> MDINDNHPTW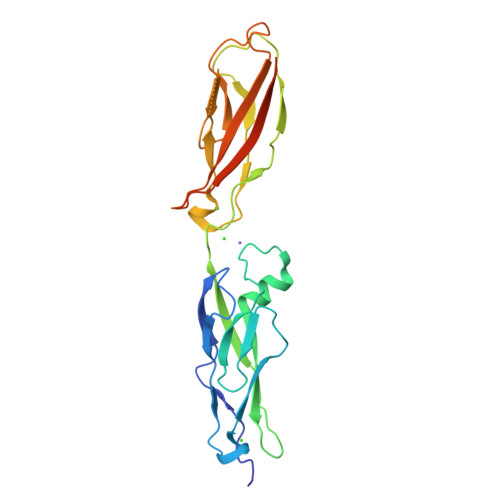KDAPYYINLVEMTPPDSDVTTVVAVDPDLGENGTLVYSIHPPNKFYSLNSTTGKIRTTHVMLDRENPDPVEAELMRKIIVSVTDCGRPPLKATSSATVFVNLLDLNDNDPTFRNLPFVAEILEGTPAGVSVYQVVAIDLDEGLNGLVSYRMQVGMPRMDFVINSTSGVVTTTAELDRERIAEYQLRVVASDAGTPTKSSTSTLTVRVLDVNDELEHHHHHH>[2x]MSEGKTEKTSHTLTKDEGFTNGGNHVPSNVTDQMTEKFDLATVYVSDAKYNRNIFFDTSPQAVKLYLLYNHWFMQTLVYVFIIINLALALFEDPAVVPLPIWATSTIETICLSAFTVRIIHYAKVIPKDKFWKDPKNICIIIIVTLSFIDMVIYGALKATGHYGIRWSRVLRPLLLVNVTEGRQLRRAFRSIRNALPQISYVFFLFMFSVLVFSLMALKLFGKRGLLTINGSPYFTDYMDIVFDLYVL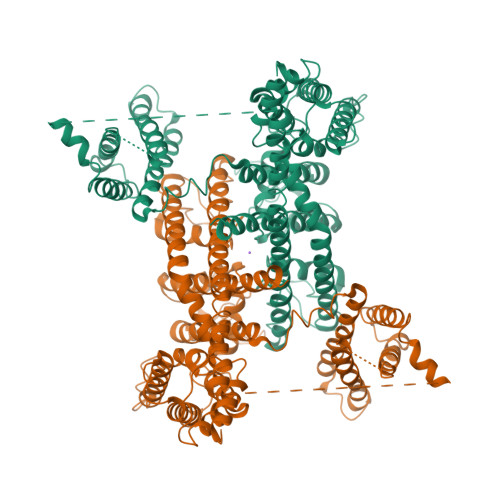VTTANSPDVMMPAYNSSVYFTIFFILYIVINTYTFMSFFLAVVYNNYKKYLKEEVRQLVKAKRIKMCRAFSLLQENRGEGGEPVVTQANWNHLVKLVKPKISTAHRELLWSVLDDQNKGHIGKFAFVQLADLLSIQVITVKSQAHPIQICFPSLYNSLPSRFIRQMVHHRVFVYAYDLIILVNAVFIGLDEENPVVSNAEWGFLALYMLEILLKLYATEPRAFFARHQFWNWFDTIIVVSALFGTIINSALKHSGGYTSRQVLDIVFILRVLRLIRVVDSIKRFRAIINTLIKIGPTILTFGQLILVVYYIFAMVGMELFKGKIQFFEPNSTSPDREYCGNPLLKSTSFAKLNYCKNNFNDVISSFILLLELTVVNQWHVLTSGFTAVTHVSARLFFVIFHIVVVIIIINIFVAFILEAFLVEYTVDKSELQTSLEKKIEELELNVQQDGVDTGLVDAMETNDSDLGSSEDGKRKPSLMFKIASRRSRTVDGLLQRMFETDLRPEDFNEEELDNTNFSNPVFDSV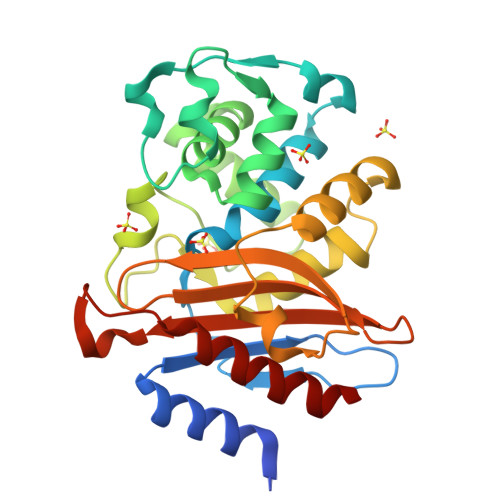>RPASTTLPAGADLADRFAELERRYDARLGVYVPATGTTAAIEYRADERFAFCSTFKAPLVAAVLHQNPLTHLDKLITYTSDDIRSISPVAQQHVQTGMTIGQLCDAAIRYSDGTAANLLLADLGGPGGGTAAFTGYLRSLGDTVSRLDAEEPELNRDPPGDERDTTTPHAIALVLQQLVLGNALPPDKRALLTDWMARNTTGAKRIRAGFPADWKVIDKTGTGDYGRANDIAVVWSPTGVPYVVAVMSDRAGGGYDAEPREALLAEAATCVAGVLA[4x]>MSSSGTPDLPVLLTDLKIQYTKIFINNEWHDSVSGKKFPVFNPATEEELCQVEEGDKEDVDKAVKAARQAFQIGSPWRTMDASERGRLLYKLADLIERDRLLLATMESMNGGKLYSNAYLNDLAGCIKTLRYCAGWADKIQGRTIPIDGNFFTYTRHEPIGVCGQIIPWNFPLVMLIWKIGPALSCGNTVVVKPAEQTPLTALHVASLIKEAGFPPGVVNIVPGYGPTAGAAISSHMDIDKVAFTGSTEVGKLIKEAAGKSNLKRVTLELGGKSPCIVLADADLDNAVEFAHHGVFYHQGQCCIAASRIFVEESIYDEFVRRSVERAKKYILGNPLTPGVTQGPQIDKEQYDKILDLIESGKKEGAKLECGGGPWGNKGYF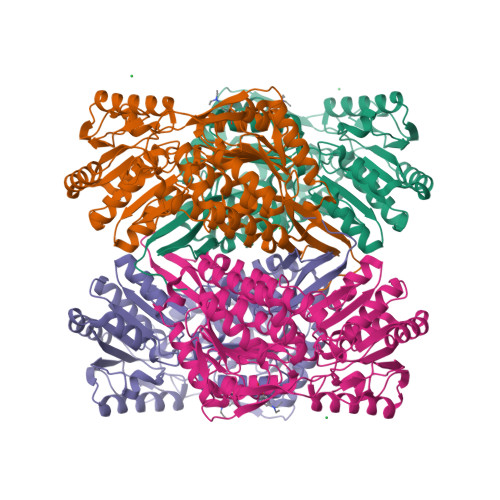VQPTVFSNVTDEMRIAKEEIFGPVQQIMKFKSLDDVIKRANNTFYGLSAGVFTKDIDKAITISSALQAGTVWVNCYGVVSAQCPFGGFKMSGNGRELGEYGFHEYTEVKTVTVKISQKNS[8x]>MVTVGNYCEAEGPVGPAWMQDGLSPCFFFTLVPSTRMALGTLALVLALPCRRRERPAGADSLSWGAGPRISPYVLQLLLATLQAALPLAGLAGRVGTARGAPLPSYLLLASVLESLAGACGLWLLVVERSQARQRLAMGIWIKFRHSPGLLLLWTVAFAAENLALVSWNSPQWWWARADLGQQVQFSLWVLRYVVSGGLFVLGLWAPGLRPQSYTLQVHEEDQDVERSQVRSAAQQSTWRDFGRKLRLLSGYLWPRGSPALQLVVLICLGLMGLERALNVLVPIFYRNIVNLLTEKAPWNSLAWTVTSYVFLKFLQGGGTGSTGFVSNLRTFLWIRVQQFTSRRVELLIFSHLHELSLRWHLGRRTGEVLRIADRGTSSVTGLLSYLVFNVIPTLADIIIGIIYFSMFFNAWFGLIVFLCMSLYLTLTIVVTEWRTKFRRAMNTQENATRARAVDSLLNFETVKYYNAESYEVERYREAIIKYQGLEWKSSASLVLLNQTQNLVIGLGLLAGSLLCAYFVTEQKLQVGDYVLFGTYIIQLYMPLNWFGTYYRMIQTNFIDMENMFDLLKEETEVKDLPGAGPLRFQKGRIEFENVHFSYADGRETLQDVSFTVMPGQTLALVGPSGAGKSTILRLLFRFYDISSGCIRIDGQDISQVTQASLRSHIGVVPQDTVLFNDTIADNIRYGRVTAGNDEVEAAAQAAGIHDAIMAFPEGYRTQVGERGLKLSGGEKQRVAIARTILKAPGIILLDEATSALDTSNERAIQASLAKVCANRTTIVVAHRLSTVVNADQI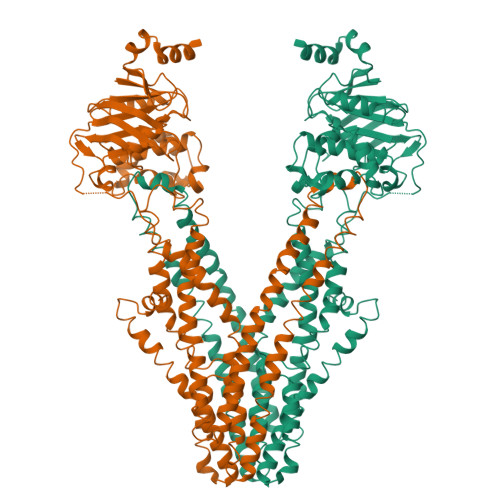LVIKDGCIVERGRHEALLSRGGVYADMWQLQQGQEETSEDTKPQTMER[2x]> MSEKSEEINEKDLRKKSELQGTALGNLKQIYYYNEKAKTENKESHDQFRQHTILFKGFFTDHSWYNDLLVRFDSKDIVDKYKGKKVDLYGAYAGYQCAGGTPNKTACMYGGVTLHDNNRLTEEKKVPINLWLDGKQNTVPLETVKTNKKNVTVQELDLQARRYLQEKYNLYNSDVFDGKVQRGLIVFHT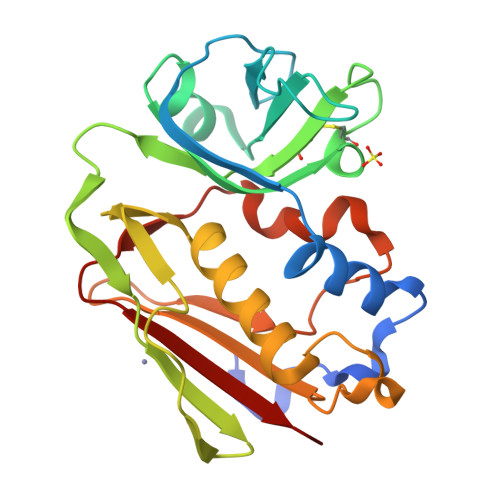STEPSVNYDLFGAQGQYSNTLLRIYRDNKTINSENMHIDIYLYTS>MKGKLTGKDKLIVDEFEELGEQESDIDEFDLLEGDEKLPGDSELDKTTSIYPPETSWEVNKGMNSSRLHKLYSLFFDKSSAFYLGDDVSVLEDKPLTGAYGFQSKKNDQQIFLFRPDSDYVAGYHVDAKSDAGWVNDKLDRRLSEISEFCSKATQPATFILPFVEMPTDITKGVQHQVLLTISYDPKSKQLTPTVYDSIGRDTYSESLSSYFKGKYRTTCDEILTQSIEKAIKSTDFTLGKFTRAAYNHQNRLTE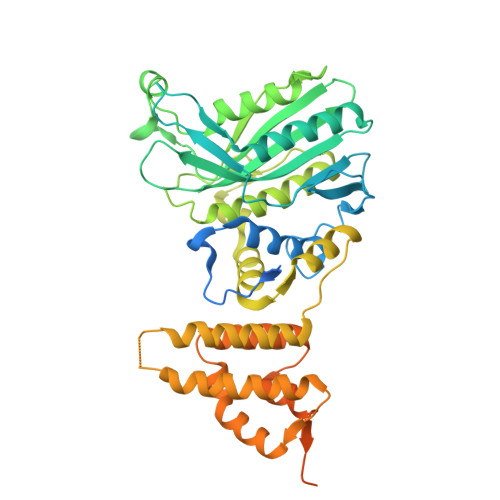GNSGSYTFRTIKEVISSSAQGTEVKIPGSGYITSNSYLTSQHVQDIESCIKYRNLGVVDIESALTEGKTLPVQLSEFIVALEDYGKLRSQQSEKSMLNFIGYSKTAKLTAVELLIGILNDIKGKNEISESQYDKLVKEVDCLMDSSLGKLVQFHLKNLGAESLQKLVLPCVKFDDTIDDFVTIEKDELFDVPDITGEELASKKGIEQGALDKEALLKQKQIKTDLLDLREEDKTGLKKPLHGGIKVK[2x]> MSGTNLDGNDEFDEQLRMQELYGDGKDGDTQTDAGGEPDSLGQQPTDTPYEWDLDKKAWFPKITEDFIATYQANYGFSNDGASSSTANVEDVHARTAEEPPQEKAPEPTDARKKGEKRKAESGWFHVEEDRNTNV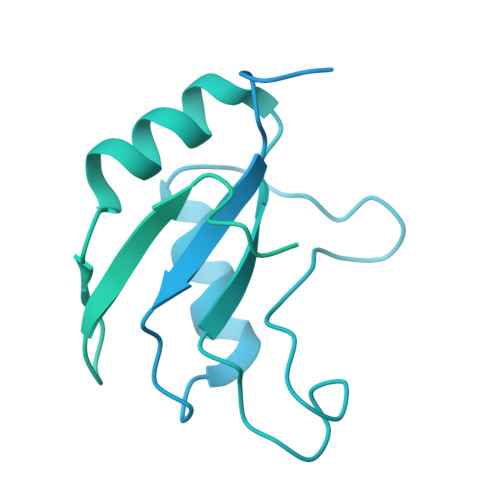YVSGLPPDITVDEFIQLMSKFGIIMRDPQTEEFKVKLYKDNQGNLKGDGLCCYLKRESVELALKLLDEDEIRGYKLHVEVAKFQLKGEYDASKKKKKCKDYKKKLSMQQKQLDWRPERRAGPSRMRHERVVIIKNMFHPMDFEDDPLVLNEIREDLRVECSKFGQIRKLLLFDRHPDGVASVSFRDPEEADYCIQTLDGRWFGGRQITAQAWDGTTDYQVEETSREREERLRGWEAFLNAPEANRGLRRSDSVSASERAGPSRARHFSEHPSTSKMNAQETATGMAFEEPIDEKKFEKTEDGGEFEEGASENNAKESSPEKEAEEGCPEKESEEGCPKRGFEGSCSQKESEEGNPVRGSEEDSPKKESKKKTLKNDCEENGLAKESEDDLNKESEEEVGPTKESEEDDSEKESDEDCSEKQSEDGSEREFEENGLEKDLDEEGSEKELHENVLDKELEENDSENSEFEDDGSEKVLDEEGSEREFDEDSDEKEEEEDTYEKVFDDESDEKEDEEYADEKGLEAADKKAEEGDADEKLFEESDDKEDEDADGKEVEDADEKLFEDDDSNEKLFDEEEDSSEKLFDDSDERGTLGGFGSVEEGPLSTGSSFILSSDDDDDDI> ACQASQLAVCASAILSGAKPSGECCGNLRAQ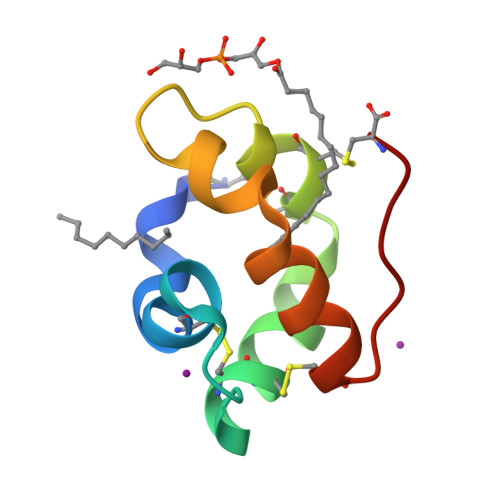QGCFCQYAKDPTYGQYIRSPHARDTLTSCGLAVPHC> MVMEDEPREATIKPSYWLDACEDISCDLIDDLVSEFDPSSVAVNESTDENGVINDFFGGIDHILDSIKNGGGLPNNGVSDTNSQINEVTVTPQVIAKETVKENGLQKNGGKRDEFSKEEGDKDRKRARVCSYQSERSNLSGRGHVNNSREGDRFMNRKRTRNWDEAGNNKKKRECNNYRRDGRDREVRGYWERDKVGSNELVYRSGTWEADHERDVKKVSGGNRECDVKAEENKSKPEERKEKVVEEQARRYQLDVLEQAKAKNTIAFLETGAGKTLIAILLIKSVHKDLMSQNRKMLSVFLVPKVPLVYQQAEVIRNQTCFQVGHYCGEMGQDFWDSRRWQREFESKQVLVMTAQILLNILRHSIIRMETIDLLILDECHHAVKKHPYSLVMSEFYHTTPKDKRPAIFGMTASPVNLKGVSSQVDCAIKIRNLETKLDSTVCTIKDRKELEKHVPMPSEIVVEYDKAATMWSLHETIKQMIAAVEEAAQASSRKSKWQFMGARDAGAKDELRQVYGVSERTESDGAANLIHKLRAINYTLAELGQWCAYKVGQSFLSALQSDERVNFQVDVKFQESYLSEVVSLLQCELLEGAAAEKVAAEVGKPENGNAHDEMEEGELPDDPVVSGGEHVDEVIGAAVADGKVTPKVQSLIKLLLKYQHTADFRAIVFVERVVAALVLPKVFAELPSLSFIRCASMIGHNNSQEMKSSQMQDTISKFRDGHVTLLVATSVAEEGLDIRQCNVVMRFDLAKTVLAYIQSRGRARKPGSDYILMVERGNVSHAAFLRNARNSEETLRKEAIERTDLS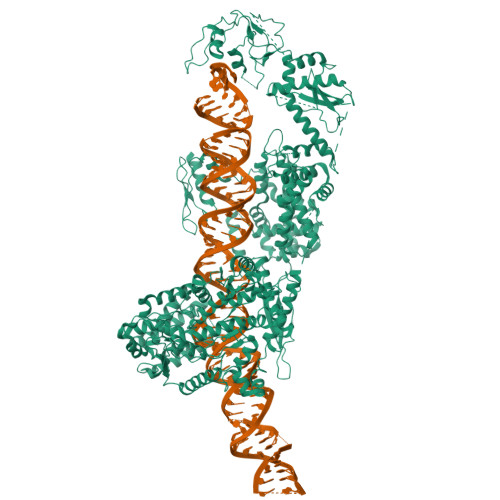HLKDTSRLISIDAVPGTVYKVEATGAMVSLNSAVGLVHFYCSQLPGDRYAILRPEFSMEKHEKPGGHTEYSCRLQLPCNAPFEILEGPVCSSMRLAQQAVCLAACKKLHEMGAFTDMLLPDKGSGQDAEKADQDDEGEPVPGTARHREFYPEGVADVLKGEWVSSGKEVCESSKLFHLYMYNVRCVDFGSSKDPFLSEVSEFAILFGNELDAEVLSMSMDLYVARAMITKASLAFKGSLDITENQLSSLKKFHVRLMSIVLDVDVEPSTTPWDPAKAYLFVPVTDNTSMEPIKGINWELVEKITKTTAWDNPLQRARPDVYLGTNERTLGGDRREYGFGKLRHNIVFGQKSHPTYGIRGAVASFDVVRASGLLPVRDAFEKEVEEDLSKGKLMMADGCMVAEDLIGKIVTAAHSGKRFYVDSICYDMSAETSFPRKEGYLGPLEYNTYADYYKQKYGVDLNCKQQPLIKGRGVSYCKNLLSPRFEQSGESETVLDKTYYVFLPPELCVVHPLSGSLIRGAQRLPSIMRRVESMLLAVQLKNLISYPIPTSKILEALTAASCQETFCYERAELLGDAYLKWVVSRFLFLKYPQKHEGQLTRMRQQMVSNMVLYQFALVKGLQSYIQADRFAPSRWSAPGVPPVFDEDTKDGGSSFFDEEQKPVSEENSDVFEDGEMEDGELEGDLSSYRVLSSKTLADVVEALIGVYYVEGGKIAANHLMKWIGIHVEDDPDEVDGTLKNVNVPESVLKSIDFVGLERALKYEFKEKGLLVEAITHASRPSSGVSCYQRLEFVGDAVLDHLITRHLFFTYTSLPPGRLTDLRAAAVNNENFARVAVKHKLHLYLRHGSSALEKQIREFVKEVQTESSKPGFNSFGLGDCKAPKVLGDIVESIAGAIFLDSGKDTTAAWKVFQPLLQPMVTPETLPMHPVRELQERCQQQAEGLEYKASRSGNTATVEVFIDGVQVGVAQNPQKKMAQKLAARNALAALKEKEIAESKEKHINNGNAGEDQGENENGNKKNGHQPFTRQTLNDICLRKNWPMPSYRCVKEGGPAHAKRFTFGVRVNTSDRGWTDECIGEPMPSVKKAKDSAAVLLLELLNKTFS> SMVSLGHLAKGASLDDLIDSCIQSFDADGNLCRSNQLLQVMLTMHRIVISSAELLQKVITLYKDALAKNSPGLCLKICYFVRYWITEFWVMFKMDASLTDTMEEFQELVKAKGEELHCRLIDTTQINARDWSRKLTQRIKSNTSKKRKVSLLFDHLEPEELSEHLTYLEFKSFRRISFSDYQNYLVNSCVKENPTMERSIALCNGISQWVQLMVLSRPTPQLRAEVFIKFIQVAQKLHQLQNFNTLMAVIGGLCHSSISRLKETSSHVPHEINKVLGEMTELLSSSRNYDNYRRAYGECTDFKIPILGVHLKDLISLYEAMPDYLEDGKVNVHKLLALYNHISELVQLQEVAPPLEANKDLVHLLTLS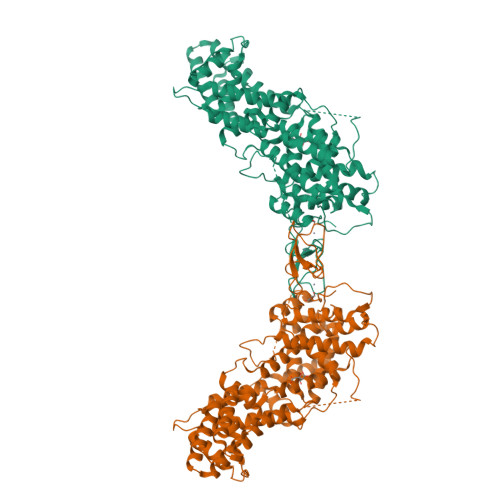LDLYYTEDEIYELSYAREPRNHRAPPLTPSKPPVVVDWASGVSPKPDPKTISKHVQRMVDSVFKNYDHDQDGYISQEEFEKIAASFPFSFCVMDKDREGLISRDEITAYFMRASSIYSKLGLGFPHNFQETTYLKPTFCDNCAGFLWGVIKQGYRCKDCGMNCHKQCKDLVVFECKKRAKNPVAPTENNTS(2R)-[(2-amino-6-oxo-6,9-dihydro-1H-purin-8-yl)sulfanyl](phenyl)acetic acid | C13 H11 N5 O3 S | 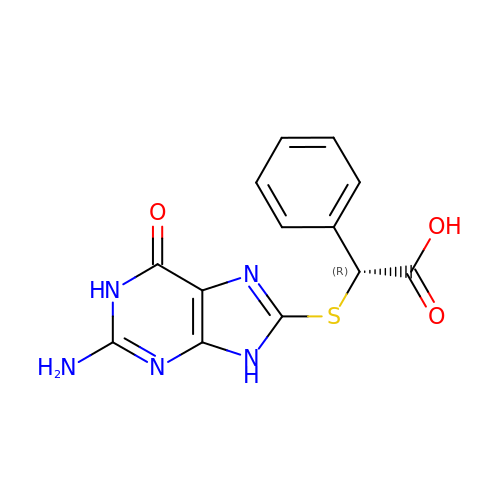CGEIBNIHDCYIDG-MRVPVSSYSA-N>[6x]GTGG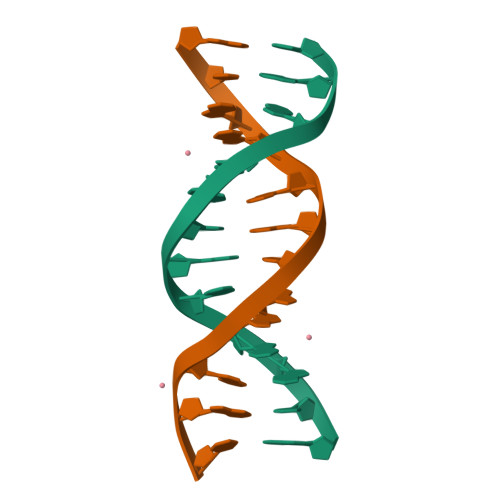AATGGAAC> ENSEVIKDLYEYLCNVRVHKSYEDDSGLWFD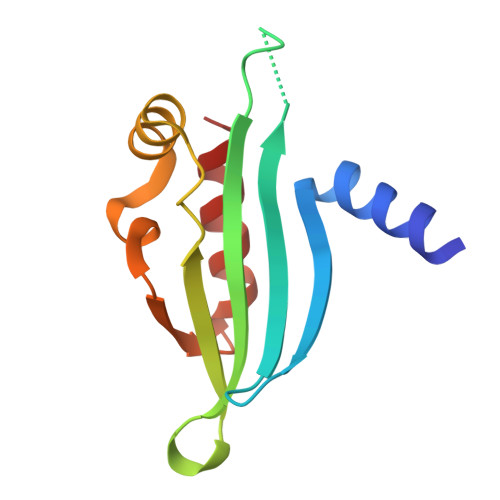ISQGTHSGGSSDDYSIMDYKLGFVKGQAQVTEVIYAPVLKQRSTEELYSLQSKLPEYLFETLSFPLSSLNQFYNKIAKSLNK METHYL HYDROGEN 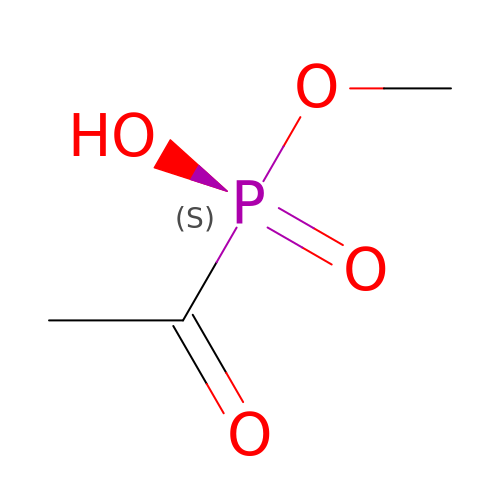(S)-ACETYLPHOSPHONATE | C3 H7 O4 P | QECABVMKPMRCRZ-UHFFFAOYSA-N> MPELPDFFEGKHFFLYGEFPGDERRRLIRYVTAFNGELEDRMNERVQFVITAQEWDPNFEEALMENPSLAFVRPRWIYSCNEKQKLLPH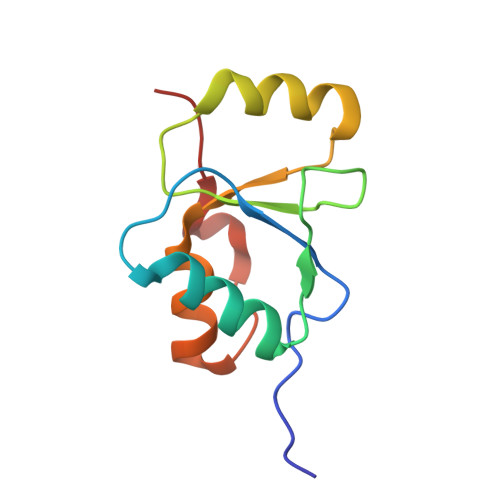QLYGVVPQA(Z)-6-(2-[2,5-DIMETHOXYPHENYL]ETHEN-1-YL)-2,4-DIAMINO-5-METHYLPYRIDO[2,3-D]PYRIMIDINE | C18 H19 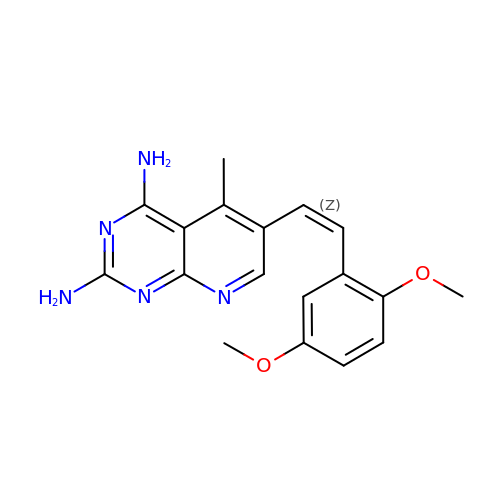N5 O2 | WNDJHUNKXPAREB-PLNGDYQASA-N> GPGETQNLNSGWTDTAHGSGIIPMRTDLELDFSLPSSASYTYRRQLQNPANEQEKIPFHLQISKQVIHAEIQHLGHWMDGTFNLKTAFHCYGSCEKYAYPWQTAGCFIEKDYEYESGWGCNPPDCPGVGTGCTACGVYLDKLKSVGKAFKIVSLRYTRKACIQLGTEQTCKSVDSNDCLVTTSVKVCLIGTVSKFQPSDTLLFLGPLEQGGLIFKQWCTTTCQFGDPGDIMSTPVGMKCPELNGSFRKKCAFATTPVCQFDGNTLSGYKRMIATKDSFQSFNVTEPHISASSLEWIDPDSSLRDHINVIVGRDLSFQDLSETPCQVDLATTSIDGAWGSGVGFNLVCSVSLTECSTFLTSIKACDSAMCYGSTTANLLRGQNTVHI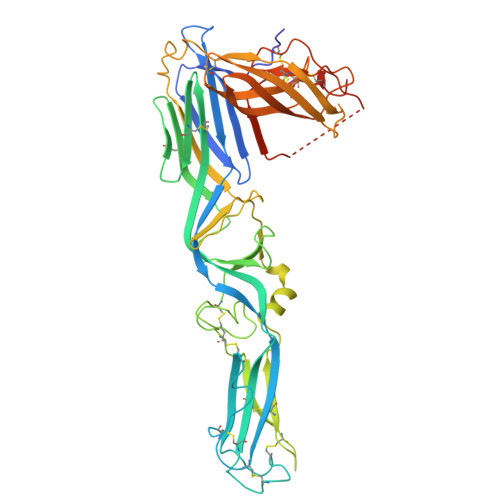VGKGGHSGSKFMCCHDTKCSSTGLVAAAPHLDRVTGYNQADSDKIFDDGAPECGISCWFTKSGEGTETSQVAPA> EAEAGNDLLSCLTFNGVRNHTVFSADSDSDFNRFLHLSIQN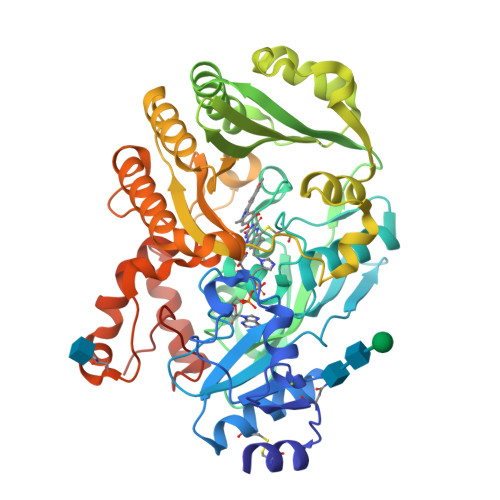PLFQNSLISKPSAIILPGSKEELSNTIRCIRKGSWTIRLRSGGHSYEGLSYTSDTPFILIDLMNLNRVSIDLESETAWVESGSTLGELYYAITESSSKLGFTAGWCPTVGTGGHISGGGFGMMSRKYGLAADNVVDAILIDANGAILDRQAMGEDVFWAIRGGGGGVWGAIYAWKIKLLPVPEKVTVFRVTKNVAIDEATSLLHKWQFVAEELEEDFTLSVLGGADEKQVWLTMLGFHFGLKTVAKSTFDLLFPELGLVEEDYLEMSWGESFAYLAGLETVSQLNNRFLKFDERAFKTKVDLTKEPLPSKAFYGLLERLSKEPNGFIALNGFGGQMSKISSDFTPFPHRSGTRLMVEYIVAWNQSEQKKKTEFLDWLEKVYEFMKPFVSKNPRLGYVNHIDLDLGGIDWGNKTVVNNAIEISRSWGESYFLSNYERLIRAKTLIDPNNVFNHPQSIPPMANFDYLEKTLGSDGGEVVI> MSLMESWLIPAAPVTVVEEIKKSRFITMLAHTD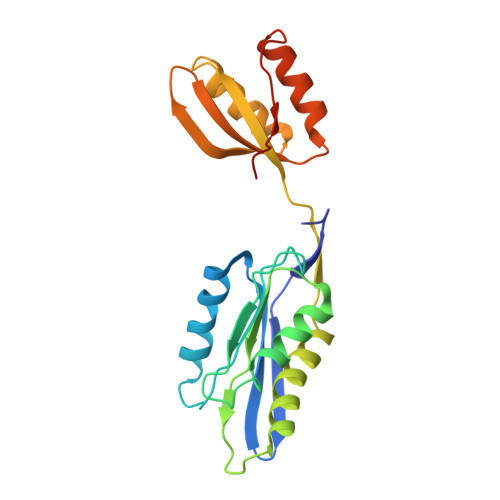GVEAAKAFVESVRAEHPDARHHCVAWVAGAPDDSQQLGFSDDGEPAGTAGKPMLAQLMGSGVGEITAVVVRYYGGILLGTGGLVKAYGGGVNQALRQLTTQRKTPLTEYTLQCEYHQLTGIEALLGQCDGKIINSDYQAFVLLRVALPAAKVAEFSAKLADFSRGSLQLLAIEEEGGSHHHHHH>[2x]ADNLAEFHVQNQECDSCHTPDGELSNDSLTYENTQCVSCHGTLAEVAETTKHEHYNAHA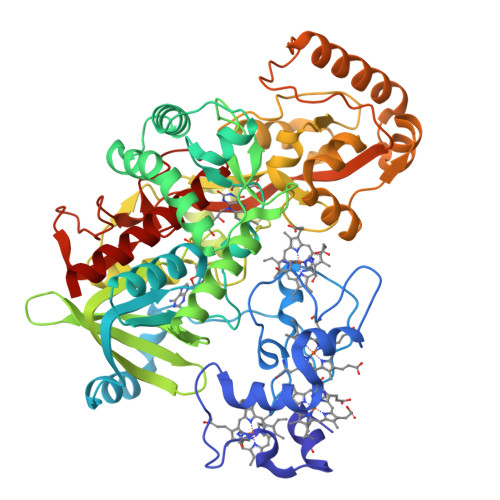SHFPGEVACTSCHSAHEKSMVYCDSCHSFDFNMPYAKKWLRDEPTIAELAKDKSERQAALASAPHDTVDVVVVGSGGAGFSAAISATDSGAKVILIEKEPVIGGNAKLAAGGMNAAWTDQQKAKKITDSPELMFEDTMKGGQNINDPALVKVLSSHSKDSVDWMTAMGADLTDVGMMGGASVNRAHRPTGGAGVGAHVVQVLYDNAVKRNIDLRMNTRGIEVLKDDKGTVKGILVKGMYKGYYWVKADAVILATGGFAKNNERVAKLDPSLKGFISTNQPGAVGDGLDVAENAGGALKDMQYIFAHPTLSVKGGVMVTEAVRGNGAILVNREGKRFVNEITTRDKASAAILAQTGKSAYLIFDDSVRKSLSKIDKYIGLGVAPTADSLVKLGKMEGIDGKALTETVARYNSLVSSGKDTDFERPNLPRALNEGNYYAIEVTPGVHHTMGGVMIDTKAEVMNAKKQVIPGLYGAGEVTGGVHGANRLGGNAISDIITFGRLAGEEAAKYSKKN> NVTPFIDVMLVLLIIFMVA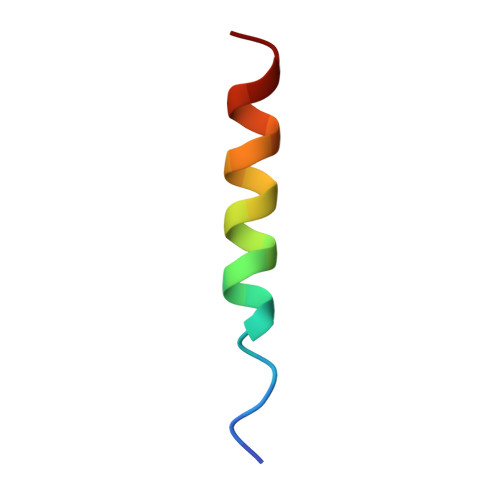APL N-[(4-methoxyphenyl)sulfonyl]-D-alanine | C10 H13 N O5 S | 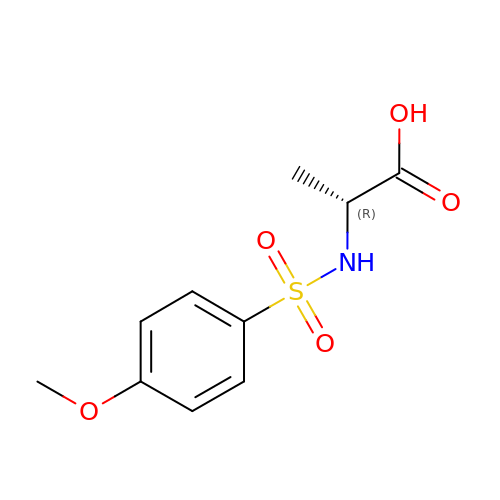XTCIPBHRVYICGT-SSDOTTSWSA-N> MRLTQGCFSFLPDLTDQQIEKQVTYAMNRGWAMNVEWTD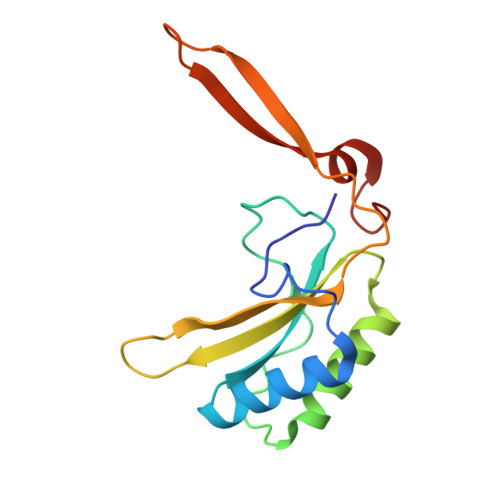DPHPRNNYWELWGLPLFDIKDPATVMFELNEARKSCAAGYIRVNAFDASYGTESCVMSFITNRPANEPGFYLDRTEGVGRQVIYSIKSYSVQANPEGSRY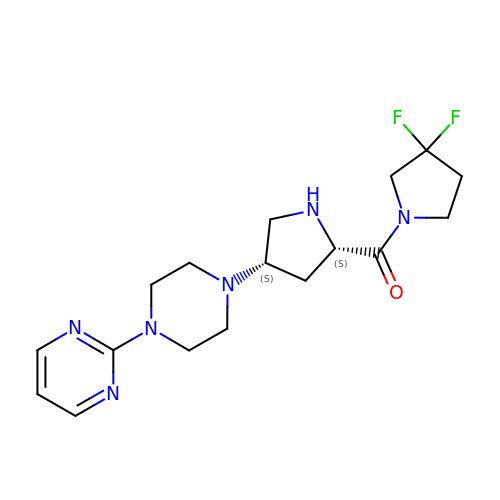2-(4-{(3S,5S)-5-[(3,3-difluoropyrrolidin-1-yl)carbonyl]pyrrolidin-3-yl}piperazin-1-yl)pyrimidine | C17 H24 F2 N6 O | QWEWGXUTRTXFRF-KBPBESRZSA-N>[2x]MVSRYVPDMGDLIWVDFDPTKGSAQAGHRPAVVLSPFMYNNKTGMCLCVPCTTQSKGYPFEVVLSGQERDGVALADQVKSIAWRARGATKKGTVAPEELQL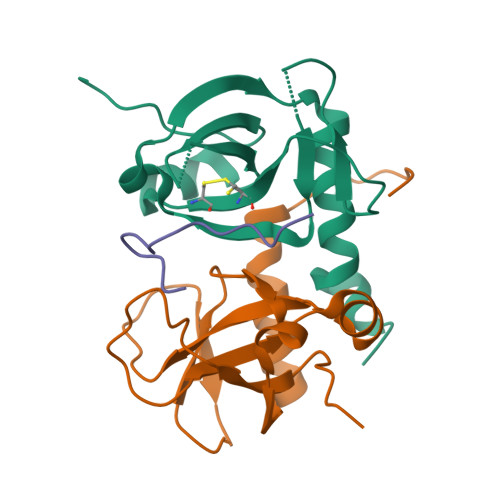IKAKINVLIGLSHHHHHH;> HENIDWGEPKDKEVW piperazine | C4 H10 N2 | 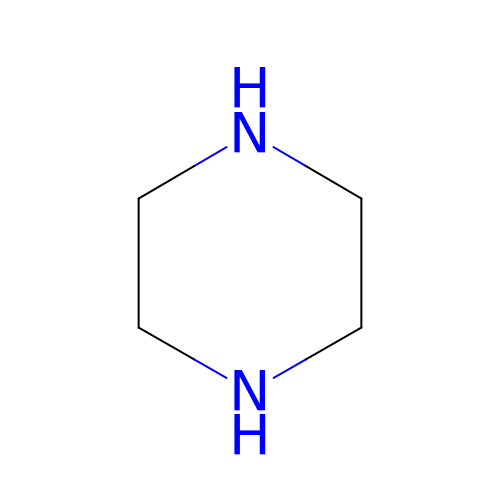GLUUGHFHXGJENI-UHFFFAOYSA-N> MHHHHHHKFRAKIVDGACLNHFTRISNMIAKLAKTCTLRISPDKLNFILCDKLANGGVSMWCELEQENFFNEFQMEGVSAENNEIYLELTSENLSRALKTAQNARALKIKLTNKHFPCLTVSVELLSMSSSSRIVTHDIPIKVIPRKLWKDLQEPVVPDPDVSIYLPVLKTMKSVVEKMKNISNHLVIEANLDGELNLK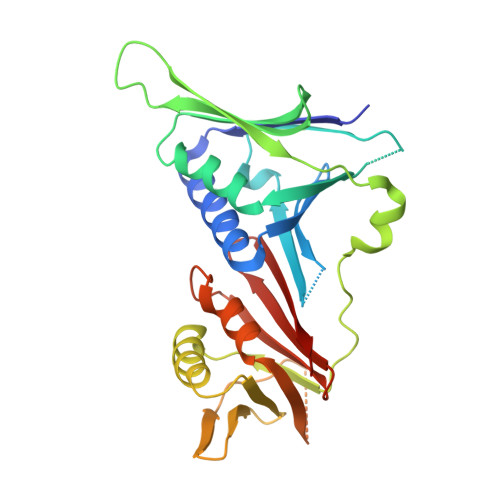IETELVCVTTHFKDLGNPPLASESTHEDRNVEHMAEVHIDIRKLLQFLAGQQVNPTKALCNIVNNKMVHFDLLHEDVSLQYFIPALS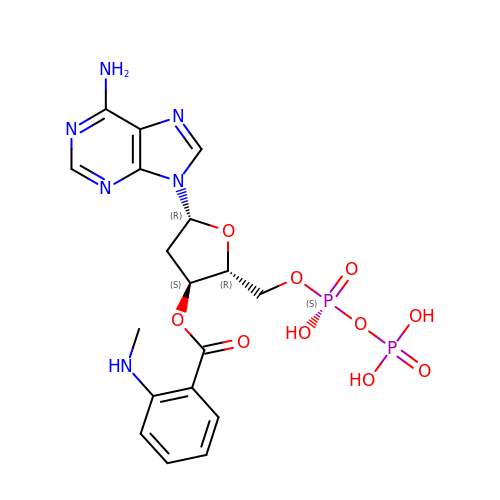2'(3')-O-N-METHYLANTHRANILOYL-ADENOSINE-5'-DIPHOSPHATE | C18 H22 N6 O10 P2 | QPKUEBLEGWBRHC-BFHYXJOUSA-N> MGGDAHAAPAEKPDPALDATKALPKALEEVEFFQSYAVRRKTGFHLFNRATGSP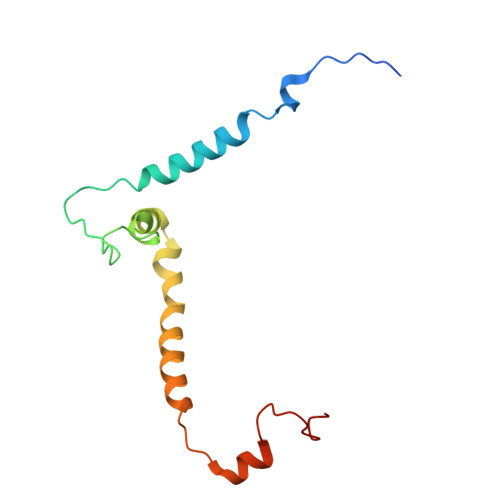TIVGPMFYNLYNFVRIGRVSKYVCWLSLPLVFQRMWMKNRATGMEYDIDLENYAPFEAKKNPMHGH>MAMHPRKDWYELTRATNWTPSYVTEEQLFPERMSGHMGIPLEKWESYDEPYKTSYPEYVSIQREKDAGAYSVKAALERAKIYENSDPGWISTLKSHYGAIAVGEYAAVTGEGRMARFSKAPGNRNMATFGMMDELRHGQLQLFFPHEYCKKDRQFDWAWRAYHSNEWAAIAAKHFFDDIITGRDAISVAIMLTFSFETGFTNMQFLGLAADAAEAGDYTFANLISSIQTDESRHAQQGGPALQLLIENGKREEAQKKVDMAIWRAWRLFAVLTGPVMDYYTPLEDRSQSFKEFMYEWIIGQFERSLIDLGLDKPWYWDLFLKDIDELHHSYHMGVWYWRTTAWWNPAAGVTPEERDWLEEKYPGWNKRWGRCWDVITENVLNDRMDLVSPETLPSVCNMSQIPLVGVPGDDWNIEVFSLEHNGRLYHFGSEVDRWVFQQDPVQYQNHMNIVDRFLAGQIQPMTLEGALKYMGFQSIEEMGKDAHDFAWADKCK[2x];>MSFESKKPMRTWSHLAEMRKKPSEYDIVSRKLHYSTNNPDSPWELSPDSPMNLWYKQYRNASPLKHDNWDAFTDPDQLVYRTYNLMQDGQESYVQSLFDQFNEREHDQMVREGWEHTMARCYSPLRYLFHCLQMSSAYVQQMAPASTISNCCILQTADSLRWLTHTAYRTHELSLTYPDAGLGEHERELWEKEPGWQGLRELMEKQLTAFDWGEAFVSLNLVVKPMIVESIFKPLQQQAWENNDTLLPLLIDSQLKDAERHSRWSKALVKHALENPDNHAVIEGWIEKWRPLADRAAEAYLSMLSSDILHAQYLERSTSLRASILTV[2x];>[2x]MSAFPVHAAFEKDFLVQLVVVDLNDS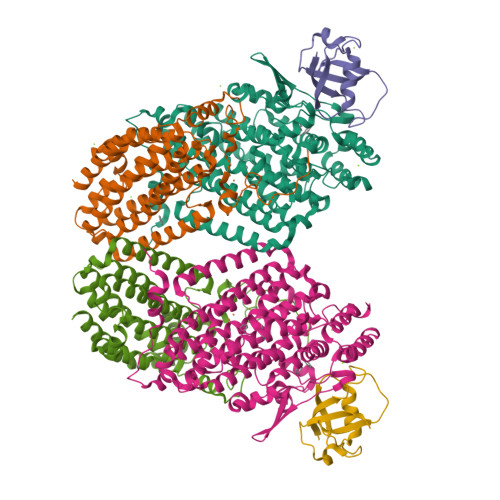MDQVAEKVAYHCVNRRVAPREGVMRVRKHRSTELFPRDMTIAESGLNPTEVIDVVFEE> GHMSKKELAAQIAEKFTDVLSKTHAEEITNFVFDHIKKALVAGKEVSIAGFGKFAVTERAARDGRNPSTGETIKIPASKSAKFKAGKQLKTDLNNN

HU proteins are the most abundant DNA-binding proteins in prokaryotic organisms and play an essential role in processes of DNA replication, repair, and recombination. HU proteins are small (approximately 90 amino acids per monomer) basic dimeric proteins that are annotated in the majority of bacteria with sequenced genomes. All HU dimers feature a compact architecture, including several intertwined α-helices, two three-stranded β-sheets, and two disordered arms that are flexible in the absence of DNA19. Recently, the HU protein from Spiroplasma melliferum KC3, an insect parasite infecting honey bees31, was produced in E. coli, purified, and crystallized, and the three-dimensional structure of this protein, referred as HUSpm, was solved at high resolution.

In the present work, we analysed the three-dimensional structure of the HU protein from the insect parasite mycoplasma S. melliferum determined at 1.4 Å resolution and found that it has unusual thermotolerance comparable to that of HU homologues from thermophilic bacteria. The monomer of recombinant HUSpm consists of 95 residues including an additional Gly-His dipeptide preceding the N-terminal Met, which was introduced by the cloning procedure. The monomer is composed of the following three canonical components: a helix-turn-helix (HTH) domain, a dimerization signal (DS) consisting of residues 48–52, and a flexible extended “arm” region — the DNA binding domain (DBD) region — responsible for DNA binding. As is seen in all known HU proteins, which are either homo- or heterodimers, the functional unit of HUSpm is a homodimer composed of two equivalent monomers (one monomer per asymmetric unit) related by a crystallographic twofold axis. Unlike other HU proteins with known three-dimensional structures, there are no salt bridges across the dimer interface in HUSpm, although a larger number of hydrogen bonds are formed compared to other HU proteins. An interesting feature of HUSpm is the presence of hydrogen bonds between the β3 and α3 regions (Lys77-Asn92 and vice versa) and between the α2 helix and the loop that links strands β1 and β2 (Gly48-Lys35 and vice versa). An analysis of the three-dimensional structure of HUSpm demonstrates that residue Phe14 of one monomer is located near Phe29 of the other monomer, which is favourable for the strengthening of the hydrophobic contact. In HUSpm, this cavity is also absent, which may be attributed to the amino acid substitution at position 31. The non-conserved Phe14 and Phe29 residues contribute to strengthening the hydrophobic dimer contact, the semi-conserved Phe31 is responsible for the absence of the internal cavity at the dimer interface, and the Lys35 and Asn92 residues are involved in the formation of unique hydrogen bonds between the monomers.1-(4-fluorophenyl)-7-methoxy-N-{[4-(methylsulfamoyl)phenyl]methyl}-1H-pyrazolo[3,4-c]pyridine-4-carboxamide | C22 H20 F N5 O4 S | 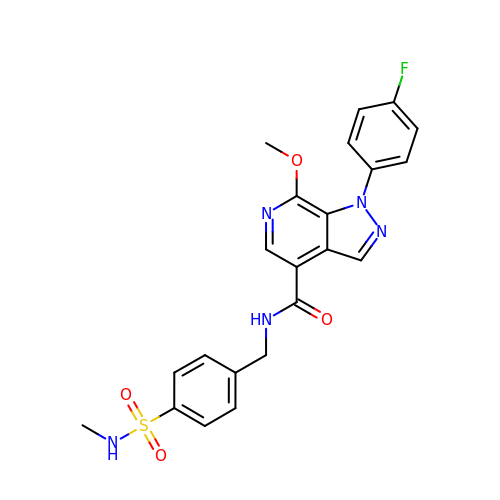XCGQNCJLJMSYMR-UHFFFAOYSA-N>MAPRKFFVGGNWKMNGDKKSLGELIHTLNGAKLSADTEVVCGAPSIYLDFARQKLDAKIGVAAQNCYKVPKGAFTGEISPAMIKDIGAAWVILGHSERRHVFGESDELIGQKVAHALAEGLGVIACIGEKLDEREAGITEKVVFEQTKAIADNVKD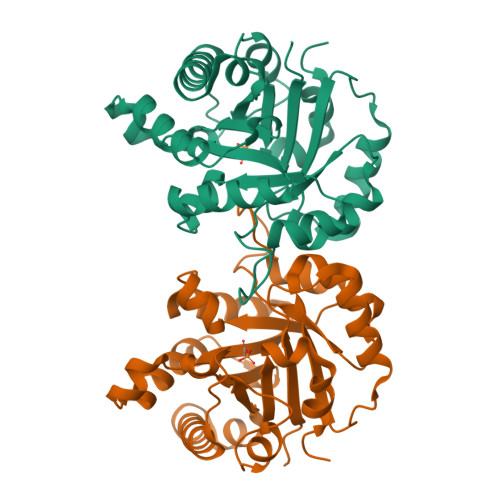WSKVVLAYEPVWAIGTGKVATPQQAQEVHEKLRGWLKSHVSDAVAQSTRIIYGGSVTGGNCKELASQHDVDGFLVGGASLKPEFVDIINAKH[2x]>RSELRFDPGTSNRNFRIAASDFGQALMLPRLYATLEETAPQVRVTGVNLRHGPLVEELESGSIDIAFGGFPTLSAGIKTQTLFREEYVCVMRQSHPALTHGLDLEAFRQCRHIIVTAHEFNHVHEQVEARLLELLPPESIRFTTENFLVSAVIAEETDVILTIPSRLARWFANRGGLTIFPVPIELPSIEVKQYWHERYDKDPGNIWLRRVIAKIGFQNPPAE[4x]

PcpR and TcpR belong to the LysR transcriptional regulator (LTTR) and are responsible for controlling the degradation of PCP and 2,4,6-TCP, respectively, although their precise mechanism of transcriptional control is not well defined. In general, the LysR family transcription factors consist of an N-terminal DNA-binding domain (DBD) and a C-terminal inducer-binding domain (IBD). The monomeric structure of the PcpR inducer-binding domain contains two nucleotide-binding (or Rossmann fold) motifs connected by a hinge region. The PcpR dimer was established by interactions between β-strands and α-helices from each monomer.

Purified recombinant PcpR protein, which covered the substrate-binding domain (residues from 85 to the C-terminus of PcpR), was crystallized in the R3 space group with 4 molecules per asymmetric unit and solved at 2.7, 2.2 and 1.9 Å resolution for the apo-form, PCP and 2,4,6-TCP binary complexes, respectively. Although 4 molecules were seen in the asymmetric unit, PcpR appears to exist as dimers in solution as illustrated by multi-angle light scattering (MALS) consistent with weak interaction between the two dimers in the crystal lattice. To further analyze the biological relevance of the oligomeric state of PcpR observed in the crystal lattice, the apo-form coordinates were uploaded to the Protein Interfaces, Surfaces, and Assemblies server (PISA). The results of PISA analysis gave average buried surface area of 1985.3 Å2 and ΔG of dimer formation to be −10.1 kcal/mol. Examination of another interface, could establish a potential tetramer, gave an average buried surface area of 254.1 Å2, ΔG of interface formation to be −0.25 kcal/mol, and CSS of 0. Overall PISA results suggested the observed dimer to be biologically relevant, but not for tetramer. Thus, the observed tetrameric nature in the asymmetric unit is likely due to crystal packing forces. A water molecule was located in all apo-form and complex structures of PcpR, forming a hydrogen bond with the backbone amide nitrogen of S104. Despite the close proximity of the PCP-binding sites in PcpR, there were no significant conformational changes of the backbone, or the dimer orientations upon comparing the apo-form to either the PCP or 2,4,6-TCP complex structures. Comparison of PcpR with BenM and DntR indicates that both our apo-form and inducer bound structures of PcpR are in the closed conformation, which could be due to a crystal packing forces.>MRGLAVLVLLVFAVQVAAAEDFRPVVFVHGLAGSAGQFESQGMRFAANGYPAEYVKTFEYDTISWALVVETDMLFSGLGSEFGLNISQIIDPETLDKILSKSRERLIDETFSRLDRVIDEALAESGADKVDLVGHSMGTFFLVRYVNSSPERAAKVAHLILLDGVWGVDAPEGIPTLAVFGNPKALPALGLPEEKVVYNATNVYFNNMTHVQLCTSPETFAVMFEFINGYKPATTDIVPQDGDYVKVKGKFLAFATNGDVSGWLSIYPIDENGKRLTRLPVKFMRVKGDFEVRLRKGQLYEFQFR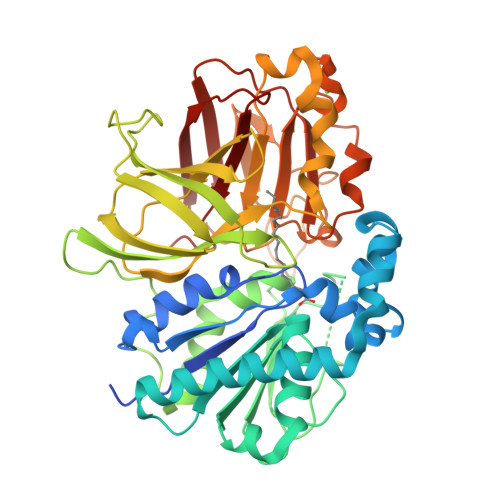KDFSPIIYHYYRAPFVRDDLWARFLVSKPPLDVELLILPERLSPAAKETSGLLLIRYKEMIGEYDEEIGGVDEVYVNGVNVCTERICPIERAVNGLWVFDRGADGKSDLDREVVRYSIMPFMSAADLVVPAEGTISIAVKSRTGGEESFTIPAWSADRHSIIVQFSDYIV[2x]> MSPPALLRASGVLLDKSMFAAKRRVIVPIQPTPGYPAHFIKTSFTTDPLKEKQKARFSSGGDAMREVQ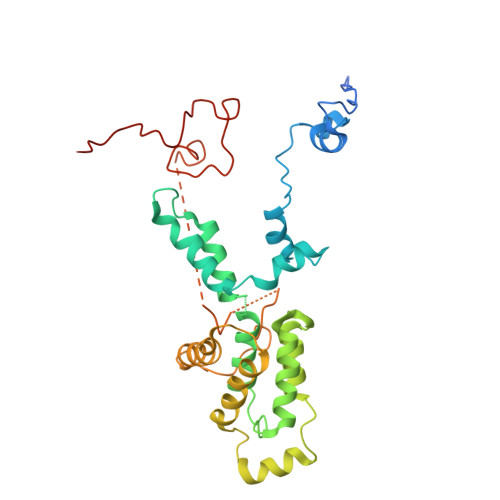DIPKRLEGQRSRAELTSRGDEDFAALIEFIQGASYDQLISGRRFRKVYEKLSENDDMFVWLCHTAMAVLNPGDMRSRLIHNHLKALAEAVASGEMTQRTAFRFFESAVRSPAYREIAARQLETGTATRLAGLAAAADVMREMGLTRRPMSSYFELYQRIVERSEAMTPWGFPPLFQFEERLALEPRLKFFSRVGQQQLERRRRGSIFSPHTILQGRRIFWIPPTWNRAGRFIGPHINLYPGLTPD>GFGCNGPWSEDDMKC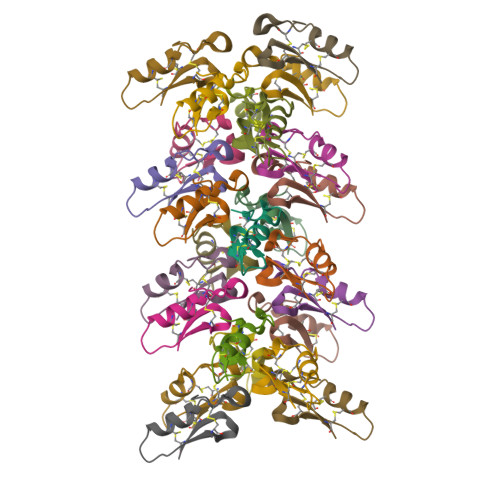HNHCKSIKGYKGGYCAKGGFLCKCY[25x]>MSSLNQLVSGLASGAVRIVDLTHTLDPDFPVIVLPPEFGQCARFRMEEISAYDHRGPAWKWHNISMSEHTGTHFDAPSHWISGKDVPNGSVDEIPAEAFVGPVVVIDCSKGAAENDDFELTPEIIAGWESEHGRIPEDAWVLMRTDWSKRRGADYLNMRADGPHSPGPTPEAIRFLIEERNIRGFGTETVGTDAGQGAHYVPPYPAHYLLHGAGKYGLQCLANLDQLPATGAVLIAAPLKIKNGTGSPLRVLAMVTE[4x]

Here we present two crystal structures of LaIHA, one bound to the hydrolytic product isatinate, and one bound to benzyl benzoate, as well as the apo structure of homologous RsIHA. Together with results from enzyme kinetic analysis, the resolved structures are used to describe the molecular basis for the Mn2+-dependent mechanism of hydrolysis, showing that IHA is a true orthologue of IHB. The highly conserved Mn2+ binding site is located at the bottom of the substrate-binding pocket.

The structures of LaIHA:benzyl benzoate and LaIHA:isatinate were determined at 1.50 Å and 1.79 Å resolution, respectively, while the one of RsIHA was determined at 2.65 Å resolution. In particular, the final binding state of isatinate shows bidentate coordination to the manganese ion, and similar stacking interactions with the indole rings of Trp59, Trp61, Trp80 and Tyr204. Asp75 forms a bidentate contact in LaIHA:Benzyl benzoate and a mono-dentate electrostatic contact in the LaIHA:isatinate structures. The mono or bi-dentate coordination results in two or one water molecules as additional ligands, respectively, preserving the octahedral geometry. Additional stabilization of the moiety into the product is obtained by the deprotonation of the nucleophile OH− group by His79 to produce a carboxylate group chelating the Mn2+ as observed in the crystal structure. The strong exothermic isomerisation step (−10 kcal mol−1) yields a structure of isatinate with a strong intra-molecular H-bond between the amino and the α-carbonyl groups. This possible intermediate most likely constitutes the driving force of the reaction and traps the isatinate as a ligand to Mn2+ in its product state before it is replaced by water and released from the binding pocket.> EAIFAAPF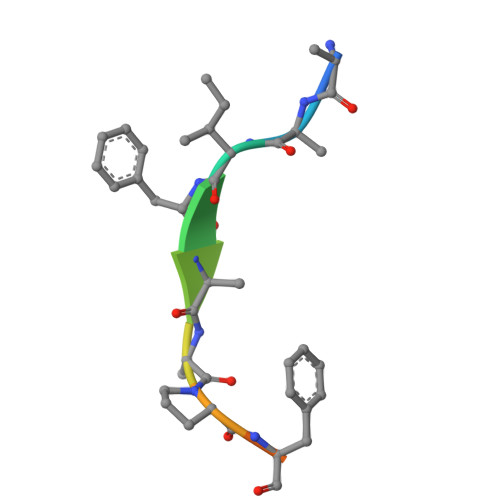AKK>MLGILNKMFDPTKRTLNRYEKIANDIDAIRGDYENLSDDALKHKTIEFKERLEKGATTDDLLVEAFAVVREASRRVTGMFPFKVQLMGGVALHDGNIAEMKTGEGKTLTSTLPVYLNALTGKGVHVVTVNEYLASRDAEQMGKIFEFLGLTVGLNLNSMSKDEKREAYAADITYSTNNELGFDYLRDNMVLYKEQMVQRPLHFAVIDEVDSILIDEARTPLIISGQAAKSTKLYVQANAFVRTLKAEKDYTYDIKTKAVQLTEEGMTKAEKAFGIDNLFDVKHVALNHHINQALKAHVAMQKDVDYVVEDGQVVIVDSFTGRLMKGRRYSEGLHQAIEAKEGLEIQNESMTLATITFQNYFRMYEKLAGMTGTAKTEEEEFRNIYNMQVVTIPTNRPVVRDDRPDLIYRTMEGKFKAVAEDVAQRYMTGQPVLVGTVAVETSELISKLLKNKGIPHQVLNAKNHEREAQIIEEAGQKGAVTIATNMAGRGTDIKLGEGVKELGGLAVVGTERHESRRIDNQLRGRSGRQGDPGITQFYLSMEDELMRRFGAERTMAMLDRFGMDDSTPIQSKMVSRAVESSQKRVEGNNFDSRKQLLQYDDVLRQQREVIYKQRFEVIDSENLREIVENMIKSSLERAIAAYTPREELPEEWKLDGLVDLINTTYLDEGALEKSDIFGKEPDEMLELIMDRIITKYNEKEEQFGKEQMREFEKVIVLRAVDSKWMDHIDAMDQLRQGIHLRAYAQTNPLREYQMEGFAMFEHMIESIEDEVAKFVMKAE[2x];>MEKLKEFLKGVRDELKRVVWPSRELVVKATISVIIFSLAIGVYLWILDLTFTKIISFILSLRGSL[2x];>MYYALLTLFVIIAVVLIISTLLQKGRGDVGAAFGGGMGQSIFGVGGVETILTKATYWLGALFLVLALLLSVIPKEKGSVVEKSVQTEQSEGKGTTQESGKGHHHHHH[2x];>[2x]MSEYLKALFELKELRQKFIFTLLMFVIYRLGSHIPIPGINPEALRDFLKAFEGSVFALYDIFSGGNLGRLTVFALGVMPYISASIMMQLLTVAIPSLQRLAKEEGDYGRYKINEYTKYLTLFVATVQ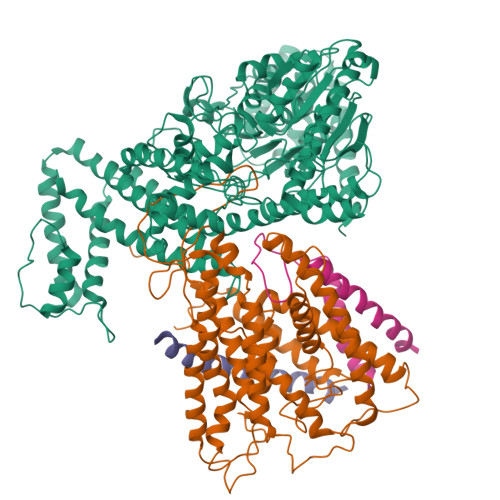SLGIAFWIRGQVSPKGIPVVENPGISFILITVLTLVAGTMFLVWIADRITEKGIGNGASLIIFAGIVANFPNAVIQFYEKVKTGDIGPLTLLLIIALIIAIIVGIVYVQEAERRIPIQYPGRQVGRQLYAGRKTYLPIKINPAGVIPIIFAQALLLIPSTLLNFVQNPFIKVIADMFQPGAIFYNFLYVTFIVFFTYFYTAVLINPVELAENLHKAGAFIPGVRPGQDTVKYLERIINRLIFFGALFLSVIALIPILISVWFNIPFYFGGTTALIVVGVALDTFRQIETYLIQKKYKSYVRR>[2x]SLRANDAPIVLLHGFTGWGREEMFGFKYWGGVRGDIEQWLNDNGYRTYTLAVGPLSSNWDRACEAYAQLVGGTVDYGAAHAAKHGHARFGRTYPGLLPELKRGGRIHIIAHSQGGQTARMLVSLLENGSQEEREYAKAHNVSLSPLFEGGHHFVLSVTTIATPHDGTTLVNMVDFTDRFFDLQKAVLEAAA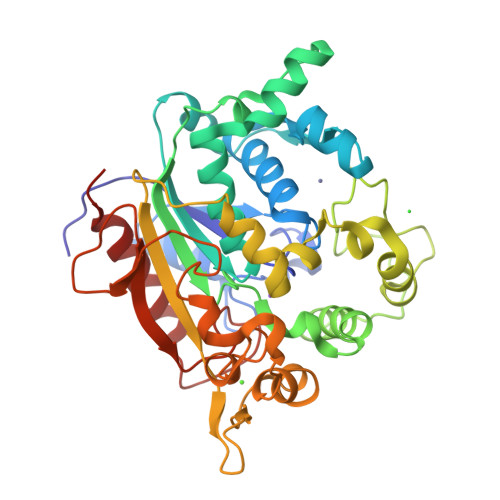VASNVPYTSQVYDFKLDQWGLRRQPGESFDHYFERLKRSPVWTSTDTARYDLSVSGAEKLNQWVQASPNTYYLSFSTERTYRGALTGNHYPELGMNAFSAVVCAPFLGSYRNPTLGIDDRWLENDGIVNTVSMNGPKRGSSDRIVPYDGTLKKGVWNDMGTYNVDHLEIIGVDPNPSFDIRAFYLRLAEQLASLQP>[2x]NDDENERSRQIDDILEKTYYNVDTHPAESLDWFNVLIGQTIQQLREEAWKKDNIVYSLNAFIERKAQELPSYLDSIKITELDIGHDFPIFSNCRIQYSPNSNGRKLEAKIDIDLNDRLAVGIETRLLLNYPKPLTASLPINVTVSIIRFQACLTVSLTKAEEF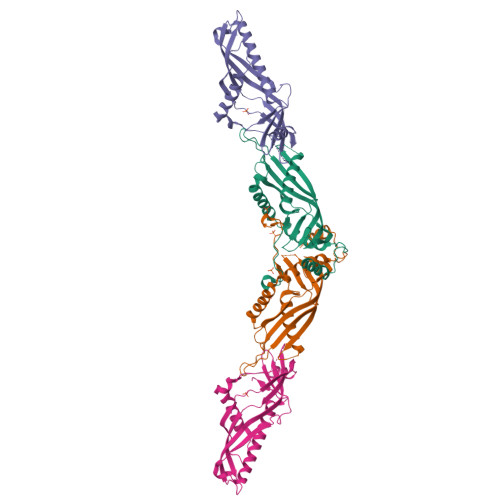VPTSPESVDEDDNDGYFLMFSFAPEYRMEFETQSLIGARSKLENIPKIGSLVEYQIKKWFVERCVEPRFQFIKLPSVWPRSKNTREGKADVD;>MSFDINWSTLESDNRLNDLIRKHLNSYLQNTQLPSYVSNLRVLDFDLGKVGPAITLKEITDPLDEFYDSIREEGGSGGSPNDIQFLLEVEYKGDLLVTIGADLVLNYPVEKFMTLPVKLSISDIGLHSLCIVACLSKQLFLSFLCDGGSIVRSMKIETEIGEQYQGQGSVLRSVGELEQFLFTIFKDFLRKELAWPSWINLDFNDGDE[2x]>KTIFVIVPTNEEQVA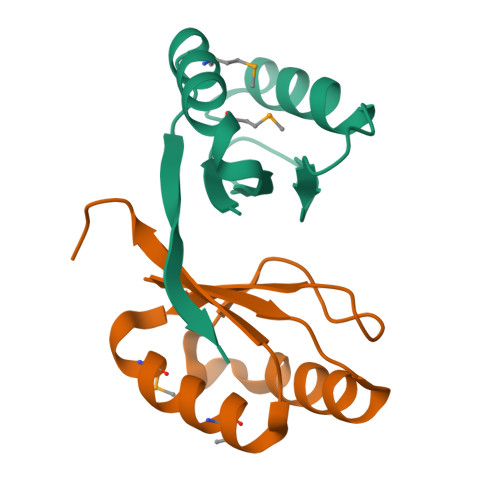FLEALAKQDELNFDWQNPPTEPGQPVVILIPSDMVEWFLEMLKAKGIPFTVYVEEGGSENKYFQ[2x]> MEEPEEPADSGQSLVPVYIYSPEYVSMCDSLAK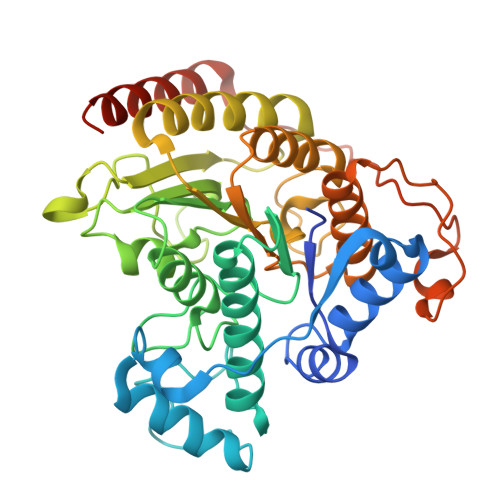IPKRASMVHSLIEAYALHKQMRIVKPKVASMEEMATFHTDAYLQHLQKVSQEGDDDHPDSIEYGLGYDCPATEGIFDYAAAIGGATITAAQCLIDGMCKVAINWSGGWAHAKKDEASGFCYLNDAVLGILRLRRKFERILYVDLDLHHGDGVEDAFSFTSKVMTVSLHKFSPGFFPGTGDVSDVGLGKGRYYSVNVPIQDGIQDEKYYQICESVLKEVYQAFNPKAVVLQLGADTIAGDPMCSFNMTPVGIGKCLKYILQWQLATLILGGGGFNLANTARCWTYLTGVILGKTLSSEIPDHEFFTAYGPDYVLEITPSCRPDRNEPHRIQQILNYIKGNLKHVVIEGRGSHHHHHH> SAIRSDFSNEDIYDNIDPDTISFPPKIATTDLFLPLFFHFGSTRQFMDKLHEVISGDYEPSQAEKLVQDLCD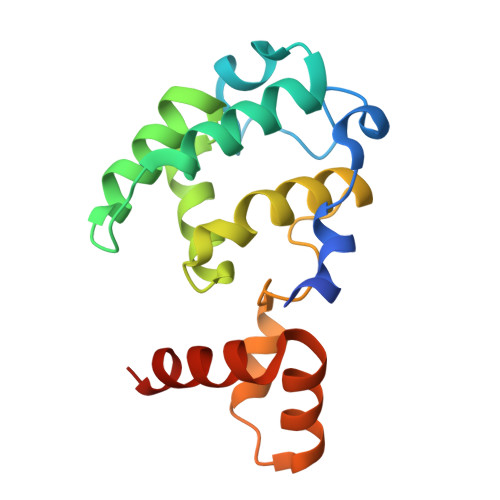ETGIRKNFSTSILTCLSGDLMVFPRYFLNMFKDNVNPPPNVPGIWTHDDDESLKSNDQEQIRKLVKKHGTGRMEMRKRFFEKDLL>[2x]MAFYSCCWVLLALTWHTSAYGPDQRAQKKGDIILGGLFPIHFGVAAKDQDLKSRPESVECIRYNFRGFRWLQAMIFAIEEINSSPALLPNLTLGYRIFDTCNTVSKALEATLSFVAQNKIDSLNLDEFCNCSEHIPSTIAVVGATGSGVSTAVANLLGLFYIPQVSYASSSRLLSNKNQFKSFLRTIPNDEHQATAMADIIEYFRWNWVGTIAADDDYGRPGIEKFREEAEERDICIDFSELISQYSDEEEIQHVVEVIQNSTAKVIVVFSSGPDLEPLI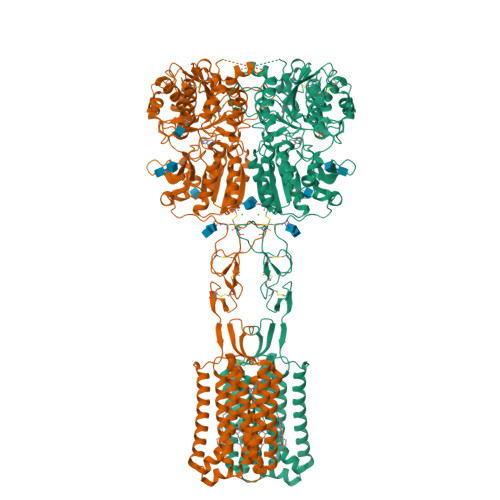KEIVRRNITGKIWLASEAWASSSLIAMPQYFHVVGGTIGFALKAGQIPGFREFLKKVHPRKSVHNGFAKEFWEETFNCHLQEGAKGPLPVDTFLRGHEESGDRFSNSSTAFRPLCTGDENISSVETPYIDYTHLRISYNVYLAVYSIAHALQDIYTCLPGRGLFTNGSCADIKKVEAWQVLKHLRHLNFTNNMGEQVTFDECGDLVGNYSIINWHLSPEDGSIVFKEVGYYNVYAKKGERLFINEEKILWSGFSREVPFSNCSRDCLAGTRKGIIEGEPTCCFECVECPDGEYSDETDASACNKCPDDFWSNENHTSCIAKEIEFLSWTEPFGIALTLFAVLGIFLTAFVLGVFIKFRNTPIVKATNRELSYLLLFSLLCCFSSSLFFIGEPQDWTCRLRQPAFGISFVLCISCILVKTNRVLLVFEAKIPTSFHRKWWGLNLQFLLVFLCTFMQIVICVIWLYTAPPSSYRNQELEDEIIFITCHEGSLMALGFLIGYTCLLAAICFFFAFKSRKLPENFNEAKFITFSMLIFFIVWISFIPAYASTYGKFVSAVEVIAILAASFGLLACIFFNKIYIILFKPSRNTIEDYKDDDDK> ATCANGKTVGDASCCAWFDVLDDIQANMFHGGQCGAEAHESIRLVFH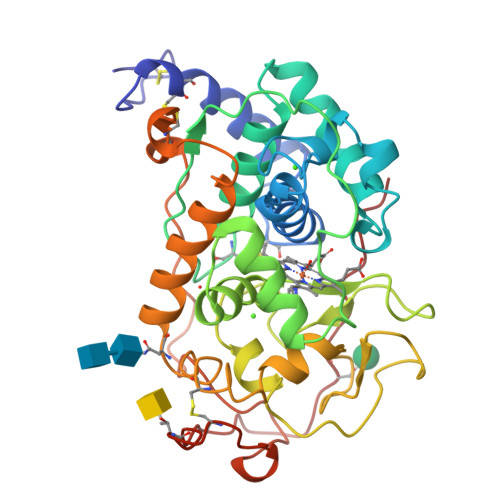DSIAISPAMEAKGKFGGGGADGSIMIFDTIETAFHPNIGLDEVVAMQKPFVQKHGVTPGDFIAFAGAVALSNCPGAPQMNFFTGRKPATQPAPDGLVPEPFHTVDQIIARVNDAGEFDELELVWMLSAHSVAAVNDVDPTVQGLPFDSTPGIFDSQFFVETQFRGTLFPGSGGNQGEVESGMAGEIRIQTDHTLARDSRTACEWQSFVGNQSKLVDDFQFIFLALTQLGQDPNAMTDCSDVIPLSKPIPGNGPFSFFPPGKSHSDIEQACAETPFPSLVTLPGPATSVARIPPHKA>GSRSELRIILVGKTGTGKSAAGNSILRKQAFESKLGSQTLTKTCSKSQGSWGNREIVIIDTPDMFSWKDHCEALYKEVQRCYLLSAPGPHVLLLVTQLGRYTSQDQQAAQRVKEIFGEDAMGHTIVLFTHK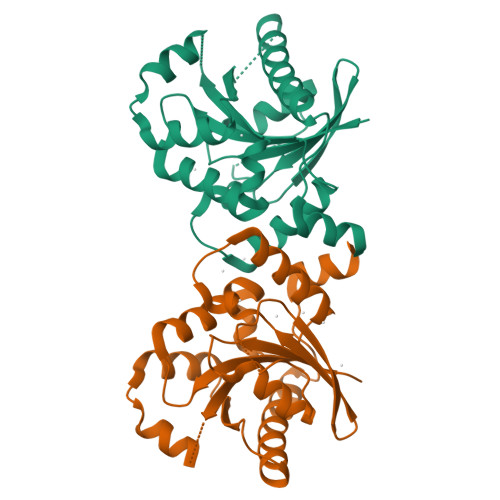EDLNGGSLMDYMHDSDNKALSKLVAACGGRICAFNNRAEGSNQDDQVKELMDCIEDLLMEKNGDHYTNGLYSLIQRSK[4x]> GAMAITMECITKKIKTIFQNSIQKCFPSISEDAIVTYANLKFGHYQCNNAINIYKKYGKELNYENAQKISEFIISNINETIFEEIKSSPQGFITVKLSKDYIETSLKKLFNGEKIDISININDIKESNENYGNVLVDFSSPNIAKEMHVGHLRSTIIGDSICRVFEFLKINTHRVNHVGDWGTQFGMIINYIKTHYPNFKEEMPDLSNLTSLYQESKKMYDADKEFEKSSKENAIKLQNNDEDCKFVWNKLCESSKKEFDKLYNILDIKLEYVGESFYVPMLSTVLDLLKESKLLTNIGDAICYQSENFKVPLFLQKSNGGYGYDSTDVAALYYRLTQLNCNCVIYVTDIGQLTHFETIFDLIKKTNWGDKNAKLMHVGFGFVLNEDNKKFKTRSGTTVKLINLIKEGTERAKRDLLQRIETKSEEEKSYFENVDIDQLSESLCVSAIKYFDLKQHRNSDYKFSYDNMLNVKGNTGIYIIYGYSRICSIFRKSTINVEDISKDELSLTSIYEINLGLHILKFPDIFYYILKNMLVHKLAEYMYDLTTTFTAFYENCKVLNNENEKSRLLLCSITKS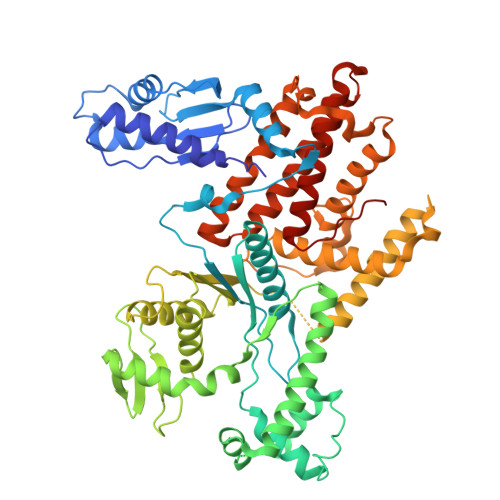LLKLCMELLGMKPIEKLENLYFQ In the development of new therapeutics, targeting the structurally similar enzymes Rv1086, Rv2361c and Rv3378c that are involved in cell-wall biosynthesis and virulence-factor production may be a possible approach. All three proteins belong to the cis-type prenyltransferase (cis-PT) family, which adopt the ζ-fold. Rv1086 produces ω,E,Z-farnesyl diphosphate (EZ-FPP; C15) from geranyl diphosphate (GPP; C10) and isopentenyl diphosphate (IPP; C5), which is used by Rv2361c for further elongation to form decaprenyl diphos­phate (DPP; C50; Kaur et al., 2004). The reaction catalyzed by Rv2361c (or M. tuberculosis DPP synthase, MtDPPS) is very similar to that of undecaprenyl diphosphate synthase (UPPS; see, for example, Ko et al., 2018), except for the chain length of the final product (C50 versus C55) and the starting allylic substrate (EZ-FPP versus EE-FPP). In fact, most cis-PTs share a common dimeric architecture, and the conserved S1 and S2 sites for substrate binding are located near the subunit interface.

Here, we report a complex structure at 1.55 Å resolution with both the S1 and S2 sites occupied by the respective allylic and homoallylic substrate analogues. One active site contained GSPP, ISPP and Mg2+, while the other only contained GSPP. Probably owing to the presence of bound substrate analogues, a previously disordered C-terminal segment became visible. The nucleophilic C4 atom of ISPP is almost collinear with the C1—S bond of GSPP, at a distance of 3.5 Å. With the cis-like positioning of the C1 and C4 atoms, the homoallylic substrate is ready to attack the allylic substrate and form a new double bond in this configuration. The Mg2+ ion forms an octahedral coordination with both phosphate groups of GSPP, the α-phosphate of ISPP, the side chain of Asp76 and two water molecules. The other has the entire molecule moved outwards, with its β-phosphate facing the solvent, its α-phosphate in the position of the β-phosphate of the first conformer and its prenyl group halfway into the tunnel. This active site contains neither an S2 ligand nor an Mg2+ ion, but the negatively charged side chain of Asp76 forms two direct hydrogen bonds to the positively charged Arg292*, which also binds to the β-phosphate in the second conformer of GSPP. Interestingly, the thiodiphosphate group of this conformer correlates well with the head group of the bisphosphonate inhibitor BPH-640 (Chan et al., 2014), suggesting that the S1 site contains a third subsite for phosphate and may be capable of triphos­phate binding. The alternative binding modes of GSPP in the magnesium-free subunit of MtDPPS, which are suggestive of a third phosphate subsite, may represent the transition state of such a translocation.

>[2x]MARDARKRTSSNFPQLPPAPDDYPTFPDTSTWPVVFPELPAAPYGGPCRPPQHTSKAAAPRIPADRLPNHVAIVMDGNGRWATQRGLARTEGHKMGEAVVIDIACGAIELGIKWLSLYAFSTENWKRSPEEVRFLMGFNRDVVRRRRDTLKKLGVRIRWVGSRPRLWRSVINELAVAEEMTKSNDVITINYCVNYGGRTEITEATREIAREVAAGRLNPERITESTIARHLQRPDIPDVDLFLRTSGEQRSSNFMLWQAAYAEYIFQDKLWPDYDRRDLWAACEEYASRTRRFGSA>ASLRANDAPIVLLHGFTGWGREEMFGFKYWGGVRGDIEQWLNDNGYRTYTLAVGPLSSNWDRACEAYAQLVGGTVDYGAAHAAKHGHARFGRTYPGLLPELKRGGRIHIIAHSQGGQTARMLVSLLENGSQEEREYAKAHNVSLSPLFEGGHHFVLSVTTIATPHDGTTLVNMVDFTDRFFDLQKAVLEAAAVASNVPYTSEVY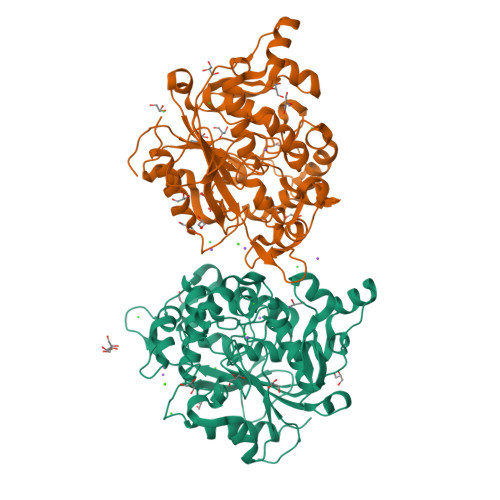DFKLDQWGLRRQPGESFDHYFERLKRSPVWTSTDTARYDLSVSGAEKLNQWVQASPNTYYLSFSTERTYRGALTGNHYPELGMNAFSAVVCAPFLGSYRNPTLGIDDRWLENDGIVNTVSMNGPKRGSSDRIVPYDGTLKKGVWNDMGTYNVDHLEIIGVDPNPSFDIRAFYLRLAEQLASLRP[2x]We reconstituted the biosynthesis of the benzoxazole moiety found in nataxazole by adding two enzymes (NatL2, NatAM), to 3‐HAA, ATP, and Mg2+. We have determined the structures of both NatL2 (homologue of BomJ) and NatAM (homologue of BomN) from the antitumor nataxazole pathway. We show NatL2 catalyzes ester not, as previously reported, amide formation; the amide is a shunt product. NatAM catalyzes benzoxazole from this ester by a mechanism that we propose involves shuttling of protons to control the fate of a hemiorthoamide intermediate.

We soaked NatL2‐AMP crystals with 3‐HAA and obtained electron density for 3‐HAA and AMP. 3‐HAA (denoted as 3‐HAA1) binds almost identically to the molecule in the AMPPNP:3‐HAA complex. There is residual electron density suggesting that we could fit a second molecule of 3‐HAA (3‐HAA2) bound adjacent to the 3‐HAA1 molecule; the orientation suggested that the hydroxyl not the amine would attack the 3‐HAA1‐adenylate. We reasoned the low quality of the residual density arose from the crowding of carboxylate of 3‐HAA1, hydroxyl of 3‐HAA2 and the α‐phosphate of AMP.

>[2x]MSRSRPELGDWSSPAELAELQRSQLPRVLAQALRSPFYAARYRGTTPPRTADDFAGVEVTAKQDLRDQYPFGMLAVGREHLATYHESSGTAGEPTASYYTEEDWTDLAERFARKWTGIHPSDTFLVRTPYGLVITGHLAQAAGRLRGATVVPGDARSLATPLSRMVRVLKTLDVTLTWCNPTEITMLAAAAKAAGLRPDQDFPHLRAMFTAAEPLTEVRRRRLSEIWGGIPVVEEYGSTETGTIAGQCPEGRMHLWADRAIFEVYDPRTGTLSEAGRGQMVVTPLYRDAMPLLRYNLADDVEVSTDPCGCGWLLPTVTVLGRAGTGHRIGPATVTQQRLEELVFSLPAAYEVMFWRAKAHPDVLELEFEAPEPVRQRAVKELGAALDRELGVPHRITGLAPGTLVPAEALTAQRDILKARYLFAEDEDWDKAVMYF> MKTEWPELVGKSVEE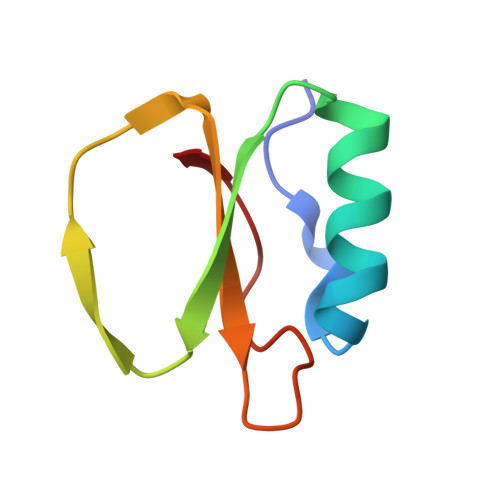AKKVILQDKPAAQIIVLPVGTIVTMEYRIDAVRLFVDRLDNIAQVPRVG> MTTTITIPNSYPIFTPNQVLTNKDLNRVVTYLDEQNRLTRVYLIGMGIVAGMEVSSIYQPGDVNIVVAPGCGITSEGYIISLAETKLTHYQSGVSVPSALFAPSEEQTAASTDQLVELFEQEGNNRLALKNLPDENAFARFLADQTLVVVYELQDQQRDSCLLDCDDTGKDRNFRLRYFLLPRSVPEKLSAEALLQQGFSREPLPQQWRDFSINDIFQAQSSFFQNFFPQVRRFGYTLETPPVIRLSNIVDYDAFLKGYQQVCLQAIDEIDRTFPNLFRLFSPFFSSFNPAPSDFTGLKTLLNQRLSDIVSGSSAENRRSPISQIEAQYALQYFYDYLSQLVSAFRELAESAFDLMDDATPDTRRFPKFLMLGL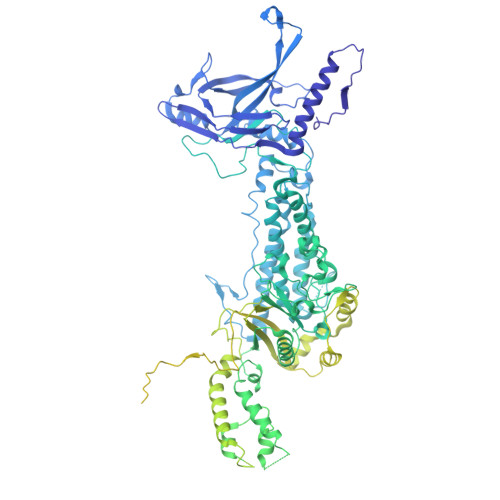VPLPNQKPEVYALNSPYRSNFSQSPIYNGNQLRVKQVRFLYDRLVRLCAADSFYLLPFYDTPLKITPSKDRAATLSQQAIPYYLNYPQLYQYWSYDTYRKGRSQSHPAYFYPNNANITPNSDLLHRLDDYSFYRIEGHIGEANATALQRILDYQQRYNLAFDVITLKIGNLQSFQDINISGQFDDLNADFGRIKDTFAKLWQRYEESWSRNVFLYTLKRVFFDKTSLAEIKSDQLFNPIVARASVKEAYEFVKESGDSYRLYLRNAAGIRIARFETVINFSGLSGDSLTQEQERIIGDLLACLPLGKITYGVEPESANNPLSYYLRFSLADELDLPANRGTADISFISLNFFTVNFEGNSPIINQPEFQDFETLYSLLRDVPESSIRVNRLELRMGDRLAADTLNYFELKGLMTAYQQRLAQIMELQLFHKFAQNNPGMEHLGGVPKGGTFVLVYVDGRELVRNLLSADRDPTYQARTEVIKKYASLPPGSPQELATSRELLNREDIVVGDFCLPYRFSSKTPTVSYVLTQPRPIVLLDRTTFCAGDETRYEFILDPTGGTLKGEGSFFADGKYYFQPSRITDDITSETAITFTYVVESSYDTLSVTVYPLPDASFQIKTNFCSNENPVTLRATQPGGNFRAFDSETDISASVINNQEFNPSAVNLGGATEKVITLVYTITSDQGCTNELSRDITIFAVPNATFQVGQGKTRFCSNDEPVDLIARVPGGTFQVRDGAEDISADVINRLTTPPQFDPSAVNLGVAREKVITLEYSISNQGCSNKFTQELRIFAVPNANFRLSTGNRDTFTNNDPPVGLIATQLGGTFQAFDGEEDITADVISPTTPPQFNPSAVNLGDEEEKVITLRYTISNQGCSNNTERRVTIVPPPEVPVRDVEDTSNPDSGDAPTENPIPHPEVRAVNLLAISNNEVINSTNLDGDRTFNLSDFNPNNQYTFEAMTVPEKVNSVIFTYTKPNGSRQALTANTAPYRMPDDWQPSIGIHEIQAQAIREVNGDRLEGATIKVIIRVIDADTDTSPSRSTNPDNLFTRIQNLFPLNRGEIITKIKLPQLLAMSTAIFMLIVGWTYSSSKQVGSTPPSVIKPR>[2x]GAMGSEPRPTAPSSGAPGLAGVGETPSAAALAAARVELPGTAVPSVPEDAAPASRDGGGVRDEGPAAAGDGLGRPLGPTPSQSRFQVDLVSENAGRAAAAAAAAAAAAAAAGAGAGAKQTPADGEASGESEPAKGSEEAKGRFRVNFVDPAASSSAEDSLSDAAGVGVDGPNVSFQNGGDTVLSEGSSLHSGGGGSGHHQHYYYDTHTNTYYLRTFGHNTMDAVPRIDHYRHTAAQLGEKLLRPSLAELHDELEKEPFEDGFANGEESTPTRDAVVTYTAESKGVVK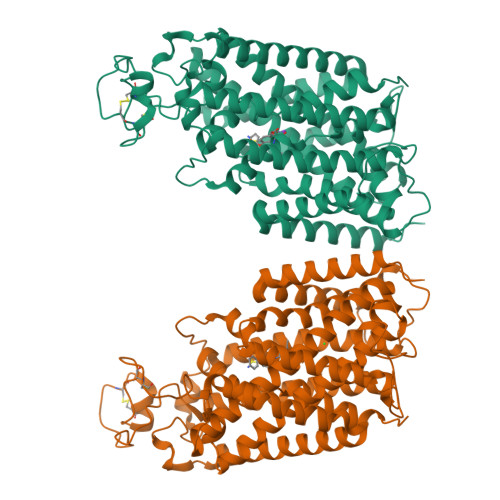FGWINGVLVRCMLNIWGVMLFIRLSWIVGQAGIGLSVLVIMMATVVTTITGLSTSAIATNGFVRGGGAYYLISRSLGPEFGGAIGLIFAFANAVAVAMYVVGFAETVVELLKEHSILMIDEINDIRIIGAITVVILLGISVAGMEWEAKAQIVLLVILLLAIGDFVIGTFIPLESKKPKGFFGYKSEIFNENFGPDFREEETFFSVFEIFFPAATGILAGANISGDLADPQSALPKGTLLAILITTLVYVGIAVSVGSCVVRDATGNVNDTIVTELTNCTSAACKLNFDFSSCESSPCSYGLMNNFQVMSMVSGFTPLISAGIFSATLSSALASLVSAPKIFQALCKDNIYPAFQMFAKGYGKNNEPLRGYILTFLIALGFILIAELNVIAPIISNFFLASYALINFSVFHASLAKSPGWRPAFKYYNMWISLLGAILCCIVMFVINWWAALLTYVIVLGLYIYVTYKKPDVNWGSSTQALTYLNALQHSIRLSGVEDHVKNFRPQCLVMTGAPNSRPALLHLVHDFTKNVGLMICGHVHMGPRRQAMKEMSIDQAKYQRWLIKNKMKAFYAPVHADDLREGAQYLMQAAGLGRMKPNTLVLGFKKDWLQADMRDVDMYINLFHDAFDIQYGVVVIRLKEGLDISHLQGQEELLSSQEKSPGTKDVVVSVEYSKKSDLDTSKPLSEKPITHKVEEEDGKTATQPLLKKESKGPIVPLNVADQKLLEASTQFQKKQGKNTIDVWWLFDDGGLTLLIPYLLTTKKKWKDCKIRVFIGGKINRIDHDRRAMATLLSKFRIDFSDIMVLGDINTKPKKENIIAFEEIIEPYRLHEDDKEQDIADKMKEDEPWRITDNELELYKTKTYRQIRLNELLKEHSSTANIIVMSLPVARKGAVSSALYMAWLEALSKDLPPILLVRGNHQSVLTFYS>SMASDSPARSLDEIDLSALRDPAGIFELVELVGNGTYGQVYKGRHVKTGQLAAIKVMDVTGDEEEEIKQEINMLKKYSHHRNIATYYGAFIKKNPPGMDDQLWLVMEFCGAGSVTDLIKNTKGNTLKEEWIAYICREILRGLSHLHQHKVIHRDIKGQNVLLTENAEVKLVDFGVSAQLDRTVGRRNTFIGTPYWMAPEVIACDENPDATYDFKSDLWSLGITAIEMAEGAPPLCDMHPMRALFLIPRNPAP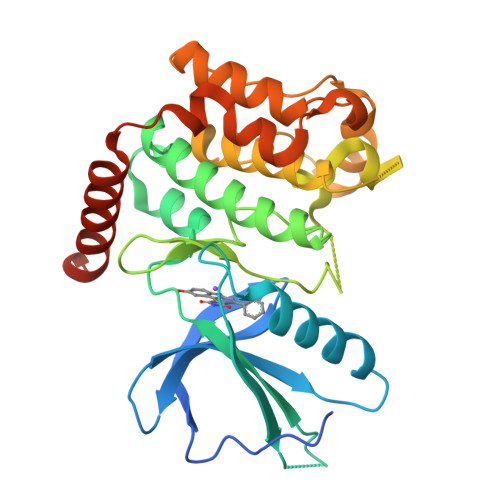RLKSKKWSKKFQSFIESCLVKNHSQRPATEQLMKHPFIRDQPNERQVRIQLKDHIDRTKKKRGEKDETEYEYSG[5x]>[14x]AVDIRDVKISFPGTQNPKFPHLRFMQTLPAVRQLTVCQRIKPFHRNTGYIFSCATSNQDNQFITSMYVKSDGTLNLGLQVNASSNKYISCPIEIELGQWYHVCH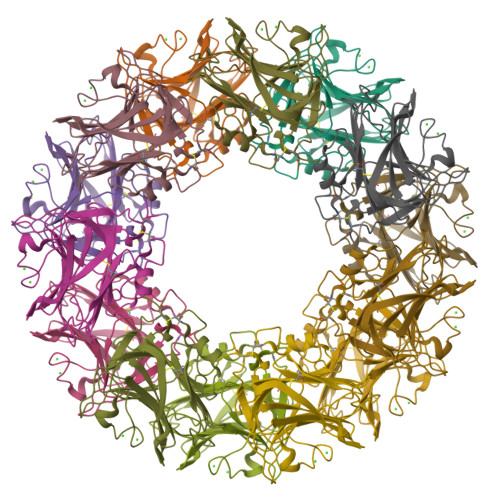VWSGVDGRMAVYANGSPCGTMENVGKGHQISAGGTVVIGQEQDKIGGGFEEQESWSGELSDLQVWDEALTTHQVSTVASCNGIRPRGNVISWMEDSFVADDGVIVGISHMCSL>[3x]MSFFHASQRDALNQSLAEVQGQINVSFEFFPPRTSEMEQTLWNSIDRLSSLKPKFVSVTYGANSGERDRTHSIIKGIKDRTGLEAAPHLTCIDATPDELRTIARDYWNNGIRHIVALRGDLPPGSGKPEMYASDLVTLLKEVADFDISVAAYPEVHPEAKSAQADLLNLKRKVDAGANRAITQFFFDVESYLRFRDRCVSAGIDVE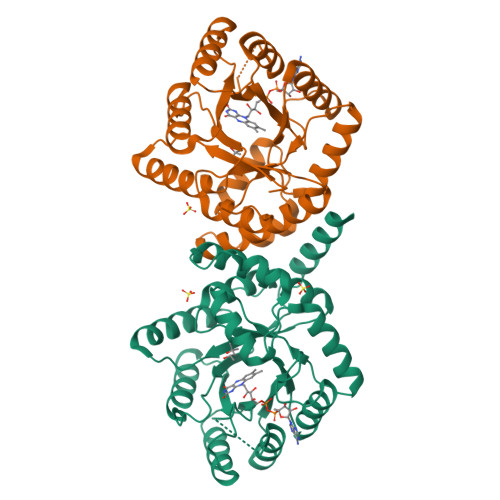IIPGILPVSNFKQAKKFADMTNVRIPAWMAQMFDGLDDDAETRKLVGANIAMDMVKILSREGVKDFHFYTLNRAEMSYAICHTLGVRPGLLEHHHHHH>[4x]SHMEQRILKFL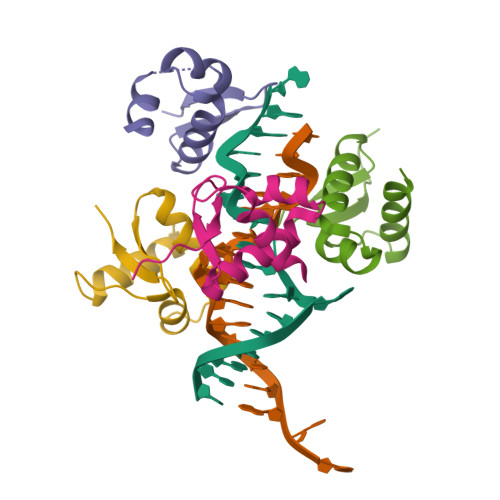EELGEGKATTAHDLSGKLGTPKKEINRVLYSLAKKGKLQKEAGTPPLWKIAVSTQ>[2x]AADWVIPPISCPENEKGEFPKNLVQIKSNRDKETKVFYSITGQGADKPPVGVFIIERETGWLKVTQPLDREAIAKYILYSHAVSSNGEAVEDPMEIVITVTDQNDNRPEFTQEVFEGSVA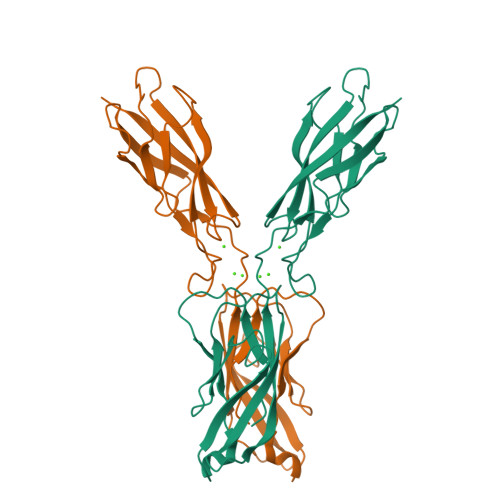EGAVPGTSVMKVSATDADDDVNTYNAAIAYTIVSQDPELPHKNMFTVNRDTGVISVLTSGLDRESYPTYTLVVQAADLQGEGLSTTAKAVITVKD> VQTKALSKATLTDLPERWENMPNLEQKEIADNLTERQKLPWKTLNNEEIKAAWYISYGEWGPRRPVHGKGDVAFITKGVFLGLGISFGLFGLV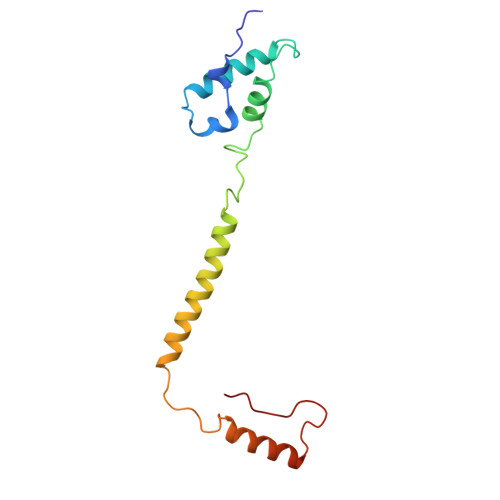RLLANPETPKTMNREWQLKSDEYLKSKNANPWGGYSQVQSK> MKSNDMNITVELTFFEPYRLVEWFDWDARKKSHSAMRGQAFAQWTWKGKGRTAGKSFITGTLVRSAVIKAVEELLSLNNGKWEGVPCCNGSFQTDESKGKKPSFLRKRHTLQWQANNKNICDKEEACPFCILLGRFDNAGKVHERNKDYDIHFSNFDLDHKQEKNDLRLVDIASGRILNRVDFDTGKAKDYFRTWEADYETYGTYTGRITLRNEHAKKLLLASLGFVDKLCGALCRIEVIKKSESPLPSDTKEQSYTKDDTVEVLSEDHNDELRKQAEVIVEAFKQNDKLEKIRILADAIRTLRLHGEGVIEKDELPDGKEERDKGHHLWDIKVQGTALRTKLKELWQSNKDIGWRKFTEMLGSNLYLIYKKETGGVSTRFRILGDTEYYSKAHDSEGSDLFIPVTPPEGIETKEWIIVGRLKAATPFYFGVQQPSDSIPGKEKKSEDSLVINEHASFNILLDKENRYRIPRSALRGALRRDLRTAFGSGCNVSLGGQILCNCKVCIEMRRITLKDSVSDFSEPPEIRYRIAKNPGTATVEDGSLFDIEVGPEGLTFPFVLRYRGHKFPEQLSSVIRYWEENDGKNGMAWLGGLDSTGKGRFALKDIKIFEWDLNQKINEYIKERGMRGKEKELLEMGESSLPDGLIPYKFFEERECLFPYKENLKPQWSEVQYTIEVGSPLLTADTISALTEPGNRAAIAYKKRVYNDGNNAIEPEPRFAVKSETHRGIFRTAVGRRTGDLGKEDHEDCTCDMCIIFGNEHESSKIRFEDLELINGNEFEKLEKHIDHVAIDRFTGGALDKAKFDTYPLAGSPKKPLKLKGRFWIKKGFSGDHKLLITTALSDIRDGLYPLGSKGGVGYGWVAGISIDDNVPDDFKEMINKTEMPLPEEVEESNNGPINNDYVHPGHQSPKQDHKNKNIYYPHYFLDSGSKVYREKDIITHEEFTEELLSGKINCKLETLTPLIIPDTSDENGLKLQGNKPGHKNYKFFNINGELMIPGSELRGMLRTHFEALTKSCFAIFGEDSTLSWRMNADEKDYKIDSNSIRKMESQRNPKYRIPDELQKELRNSGNGLFNRLYTSERRFWSDVSNKFENSIDYKREILRCAGRPKNYKGGIIRQRKDSLMAEELKV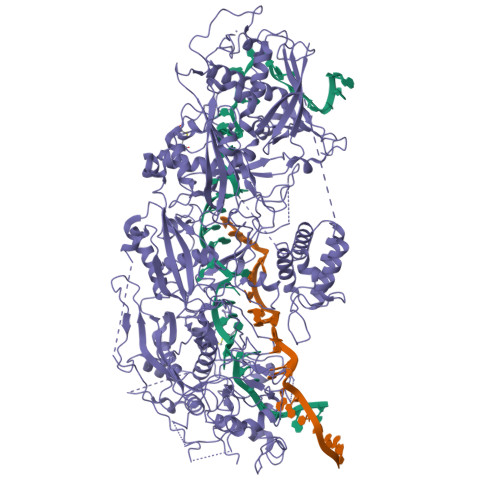HRLPLYDNFDIPDSAYKANDHCRKSATCSTSRGCRERFTCGIKVRDKNRVFLNAANNNRQYLNNIKKSNHDLYLQYLKGEKKIRFNSKVITGSERSPIDVIAELNERGRQTGFIKLSGLNNSNKSQGNTGTTFNSGWDRFELNILLDDLETRPSKSDYPRPRLLFTKDQYEYNITKRCERVFEIDKGNKTGYPVDDQIKKNYEDILDSYDGIKDQEVAERFDTFTRGSKLKVGDLVYFHIDGDNKIDSLIPVRISRKCASKTLGGKLDKALHPCTGLSDGLCPGCHLFGTTDYKGRVKFGFAKYENGPEWLITRGNNPERSLTLGVLESPRPAFSIPDDESEIPGRKFYLHHNGWRIIRQKQLEIRETVQPERNVTTEVMDKGNVFSFDVRFENLREWELGLLLQSLDPGKNIAHKLGKGKPYGFGSVKIKIDSLHTFKINSNNDKIKRVPQSDIREYINKGYQKLIEWSGNNSIQKGNVLPQWHVIPHIDKLYKLLWVPFLNDSKLEPDVRYPVLNEESKGYIEGSDYTYKKLGDKDNLPYKTRVKGLTTPWSPWNPFQVIAEHEEQEVNVTGSRPSVTDKIERDGKMV> GPGADAVDVPLIKNLYAEAWKQQYSDLRLSTKQTESCGLAANTEYIAAPWDVGGGGVLGILRLADIGRNPAVAKIKGHTASIQDTNFSPFYRDILATACEDTIVRIWQLPEEVTGTTELKEPIATLTGALKKVLSAEWNPAVSGILASGCFDGTVAFWNVEKNENFASVKFQESLLSAKWSWKGDLLACTTKDKALNIVDPRAAQVVGSVACHDGSKACKCTWIDGL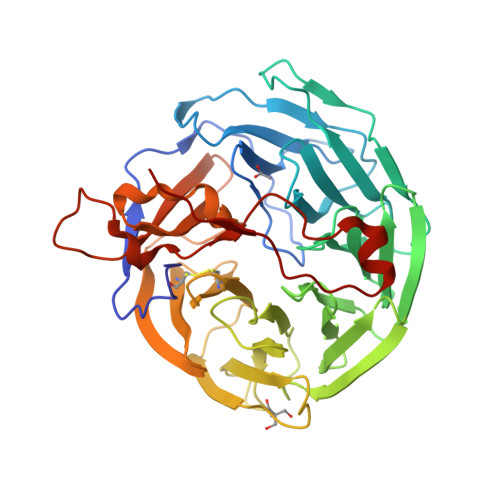AGRDGHVFTTGFGKMQEREMAIWDTRKFDKPVYHAEIDRGSSPLYPIFDETTGMLYVCGKGDSSCRYYQYHGGTLRSVDAYRSSVPIKNFCFIPKLAVDQMRAEIGRMLKQENGNVLQPISFIVPRKNQDVFQADLYPPAPDVEPSMTAEEWFKGENKAIRRRSVKP>[2x]GQFKRIALLGMPNTGKSTLFNRMTGGAARVGNWPGITVELLSGKILLGADMVEIIDLPGIYDLHGFSDDEQV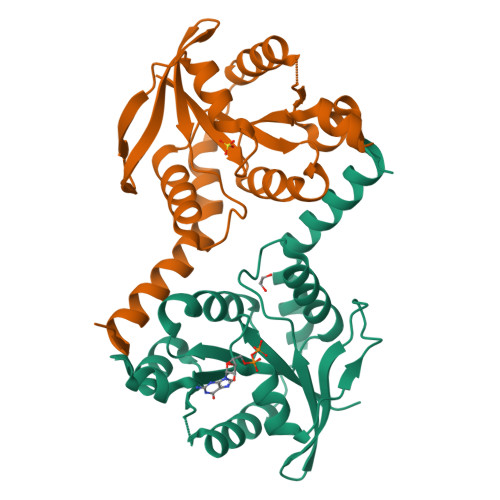VRHFLHDNVPDLALVILNATQIERQMSLLLQLKQLNMNIVVLLNMSDEAKQYGITIDSRKMSELLQIPVFQLSGKYGTGYQEALQAVTRALRYPTPGMAENVRTQLEQDEHIEAEMVRILKSAVQIPARLPE>SNVPHKSSLPEGIRPGTVLAIAGLVPPNASRFHVNLLCGEEQGSDAALHFNPRLDTSEVVFNSKEQGSWGREERGPGVPFQRGQPFEVLIIASDDGFKAVVGDAQYHHFRHRLPLARVRLVEVGGDVQLDSVR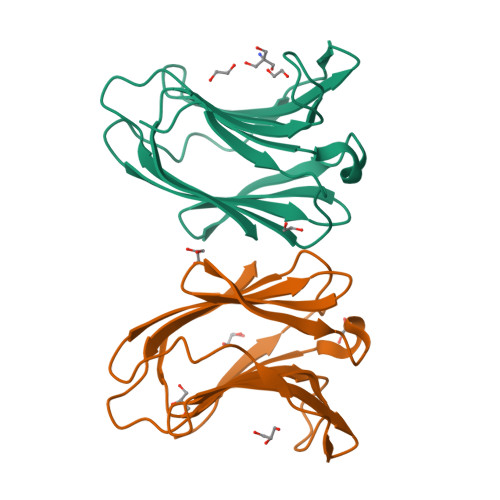IF[2x]> GAMTVFRQENVDDYYDTGEELGSGQFAVVKKCREKSTGLQYAAKFIKKRRTKSSRRGVSREDIEREVSILKEIQHPNVITLHEVYENKTDVILILELVAGGELFDFLAEKESLTEEEATEFLKQILNGVYYLHSLQIAHFDLKPENIMLLDRNVPKPRIKIIDFGLAHKIDFGNEFKNIFGTPEFVAPEIVNYEPLGLEADMWSIGVITYILLSGASPFLGDTKQETLANVSAVNYEFEDEYFSNTSAL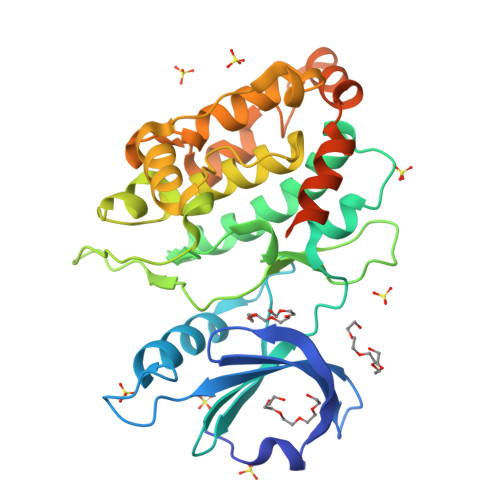AKDFIRRLLVKDPKKRMTIQDSLQHPWIKPKDTQQALSRKASAVNMEKFKKFAAAKKWKQSVRLISLCQRLSRSFLSRSNMSVARSD To counteract the mutational effects of deamination damages, a unique alternative excision repair pathway has evolved, in which the enzyme endonuclease V (EndoV) plays an important role. EcEndoV primarily incises deoxyinosine (dI) in DNA19 at the second phosphodiester bond 3′ to the lesion, producing a nick with a 3′-hydroxyl and a 5′-phosphoryl group. In addition, EcEndoV also cleaves the U, O, X, apurinic/apyrimidinic (AP) site, insertion/deletion mismatches (IDM), flaps, loops and pseudo-Y DNA structures, when Mn2+ is supplied as a metal cofactor. EcEndoV is the first member discovered in the EndoV family and it has a broad substrate spectrum.

To investigate the substrate recognition and catalytic mechanism of EcEndoV, we solved the crystal structure of apo EcEndoV. In order to obtain diffraction-quality crystals, the 9-residue, C-terminal fragment was truncated. The resultant construct is prone to aggregation, but still retains the deoxyinosine-specific endonuclease activity (data not shown). This construct contains residues M1-A214 (named EcEndoV-SF) and it forms plate crystals in a condition containing PEG 3350. The crystals belong to an orthorhombic system with the space group P212121, and each asymmetric unit contains two monomers. Both chains are almost completely intact with no internal disorders and of good electron density: chain A is visible from M1-V208 and chain B is visible from M1-S210. The enzyme displays the ‘RNase H-like motif’. Two of the most important elements for substrates binding and recognition are the PYIP motif consisting of residues P72, Y73, I74 and P75, and the hypoxanthine-binding pocket comprising hydrophobic residues Y73, P75, and L78 and V115 (corresponding to I122 in TmEndoV). Additionally, four conserved glycines G76, G104, G106 and G114 also participate in the formation of the rigid pocket and their backbone atoms are involved in hypoxanthine recognition. No Mg2+ is found at the cleavage site. The r.m.s. deviation is 1.4 Å over 204 Cα atoms between EcEndoV-SF and apo TmEndoV.

>[2x]GPHMDLASLRAQQIELASSVIREDRLDKDPPDLIAGADVGFEQGGEVTRAAMVLLKYPSLELVEYKVARIATTMPYIPGFLSFREYPALLAAWEMLSQKPDLVFVDGHGISHPRRLGVASHFGLLVDVPTIGVAKKRLCGKFEPLSSEPGALAPLMDKGEQLAWVWRSKARCNPLFIATGHRVSVDSALAWVQRCMKGYRLPEPTRWADAVASERPA>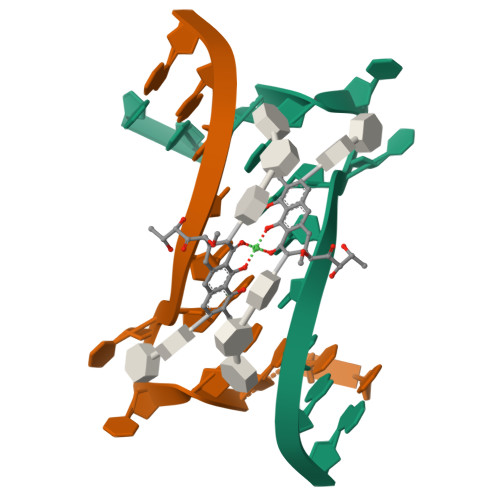[2x]TTCCGCCGCCGAA> MDPYYPFDALDVWEHRRFIVADSRSFITPEFPRDFWMLPVFNIPRETAAERAAVLQAQRTAAAAALENAALQAAELPVDIERRIRPIEQQVHHIADALEALETAAAAAEEADAARDAEARGEGAADGAAPSPTAGPAAAEMEVQIVRNDPPLRYDTNLPVDLLHMVYAGRGAAGSSGVVFGTWYRTIQERTIADFPLTTRSADFRDGRMSKTFMTALVLSLQSCGRLYVGQRHYSAFECAVLCLYLLYRTTHESSPDRDRAPVAFGDLLARLPRYLARLAAVIGDESGRPQYRYRDDKLPKAQFAAAGGRYEHGALATHVVIATLVRH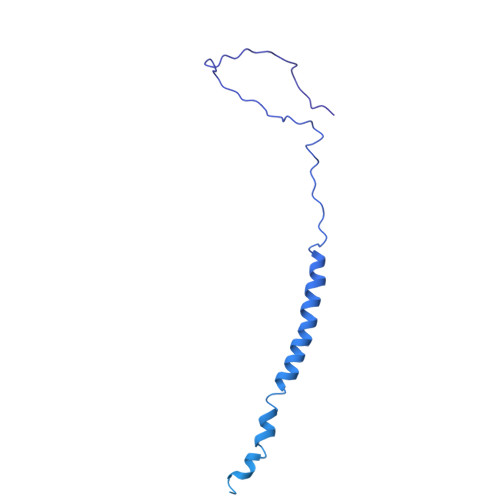GVLPAAPGDVPRDTSTRVNPDDVAHRDDVNRAAAAFLARGHNLFLWEDQTLLRATANTITALAVLRRLLANGNVYADRLDNRLQLGMLIPGAVPAEAIARGASGLDSGAIKSGDNNLEALCVNYVLPLYQADPTVELTQLFPGLAALCLDAQAGRPLASTRRVVDMSSGARQAALVRLTALELINRTRTNTTPVGEIINAHDALGIQYEQGPGLLAQQARIGLASNTKRFATFNVGSDYDLLYFLCLGFIPQYLSVA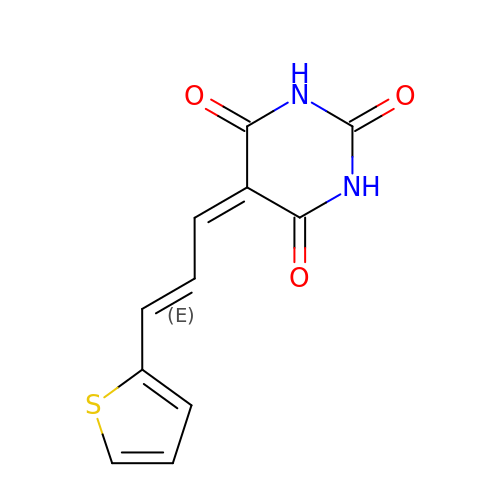5-[(E)-3-thiophen-2-ylprop-2-enylidene]-1,3-diazinane-2,4,6-trione | C11 H8 N2 O3 S | XVDGTYMDHFXORY-HNQUOIGGSA-N>[2x]MNDTAGELEFVPLAANDDETVGQWLDLMALAAETGPRAAPPCNVDMVGSLRFAPPATALDDWVVRSGGRVVGALRLALPDGAPTARV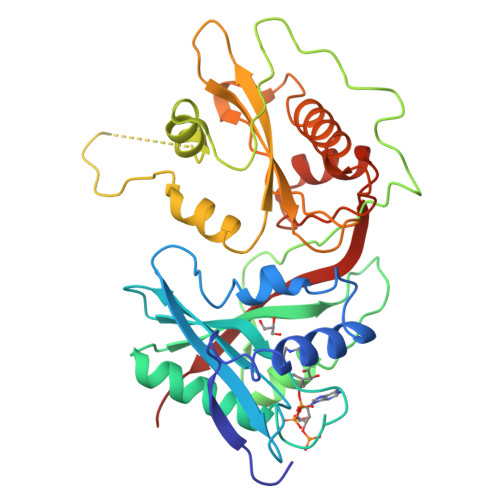DQLLVHPGRRRRGIGRALWAHARELARKHDRTTLTATVVESLPSGPAQDPGPAAFAAAMGAHRSDIPAGTHQWLDLDRHDPLADGVPAVPAGYSLVTWGTITPDEYAVPVSELELSLGAGPVDRAAQEVRTSYARQFETMRVGRGRRAYHTGAVHDATGALAGYTSVSKTTGNPAYALQGMTVVHREHRGHALGTLLKLANLEYVLRHEPEVRLVETANAEDNHPMIAVNAALGFEPYDRWVFWTAEAGPSD> YVDYKDDDDKEVEVCSEQAEVGPCRARFSRWYFDVTEGKCAPFVYGGCGGNRNNF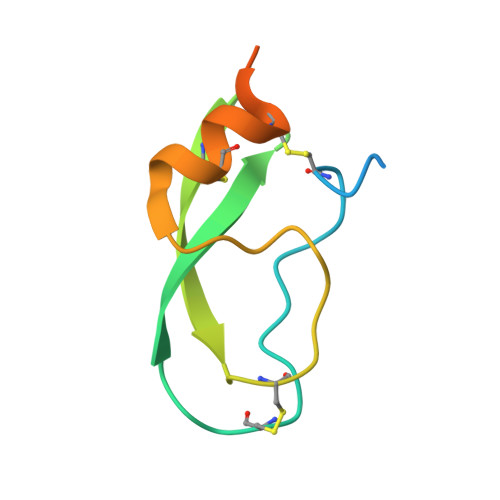DTEEYCMAVCGSAIPRHHHHHHAAAN>[3x]MSGSYDEASEEITDSFWEVGNYKRTVKRIDDGHRLCNDLMSCVQERAKIEKAYAQQLTDWAKRWRQLIEKGPQYGSLERAWGAMMTEADKVSELHQEVKNSLLNEDLEKVKN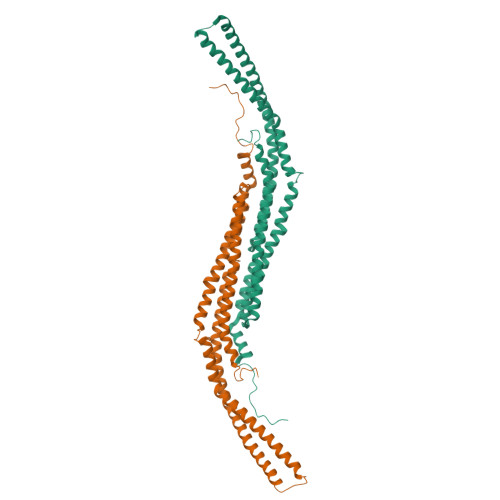WQKDAYHKQIMGGFKETKEAEDGFRKAQKPWAKKMKELEAAKKAYHLACKEERLAMTREMNSKTEQSVTPEQQKKLVDKVDKCRQDVQKTQEKYEKVLEDVGKTTPQYMEGMEQVFEQCQQFEEKRLVFLKEVLLDIKRHLNLAENSSYMHVYRELEQAIRGADAQEDLRWFRSTSGPGMPMNWPQFEEWNPDLPHTTAKKEKQPKKAEGATLSNATGAVESTSQ> MHLMRACITFCIASTAVVAVNAALVAEDAPVLSKAFVDRVNRLNRGIWKAKYDGVMQNITLREAKRLNGVIKKNNNASILPKRRFTEEEARAPLPSSFDSAEAWPNCPTIPQIADQSACGSCWAVAAASAMSDRFCTMGGVQDVHISAGDLLACCSDCGDGCNGGDPDRAWAYFSSTGLVSDYCQPYPFPHCSHHSKSKNGYPPCSQFNFDTPKCNYTCDDPTIPVVNYRSWTSYALQGEDDYMRELFFRGPFEVAFDVYEDFIAYNSGVYHHVSGQYLGGHAVRLVGWGTSNGVPYWKIANSWNTEWGMDGYFLIRRGSSECGIEDGGSAGIPLAPNTA

The crystal structure of Trypanosoma brucei procathepsin B (TbCatB) in complex with its native propeptide represents the first novel bioinformation obtained by applying the SFX approach at a free-electron laser. This enzyme is of scientific and medical interest, since the knockout of its encoding gene has been shown to be lethal to the parasite that causes sleeping sickness in Africa, which turns TbCatB into an urgently required potential new drug target. TbCatB crystals grew spontaneously within living baculovirus-infected insect cells during protein overexpression to a size of 10–15 µm in the longest dimension.

By combining diffraction data from 80 Trypanosoma brucei procathepsin B crystals with an average volume of 9 µm3, a complete data set to 3.0 Å resolution has been assembled. Diffraction experiments were conducted on the P14 microfocus beamline at the PETRA III storage ring (DESY, Hamburg) with a 4 × 5 µm (FWHM) microfocus beam, a total photon flux of 1.2 × 1012 photons s−1 at the sample position and a photon energy of 10.00 keV. To collect a complete data set, we employed a data-collection strategy in which a region of interest of 600 × 600 µm was raster scanned with rotation exposures. After iterative merging and scaling, 109 661 reflection intensities in the resolution range from 88 to 3.0 Å were merged into a final data set consisting of 8881 merged reflection intensities with an overall completeness of 99.8%. This final set of reflection intensities included data from 426 diffraction patterns collected from 80 individual TbCatB crystals in 120 groups. During stepwise model building and refinement, 62 propeptide residues and five carbohydrate residues were manually placed in difference electron-density maps. No electron density is observed for nine flexible amino-acid side chains mainly located within a loop region spanning residues His195–Asn209 or for ten atoms of the carbohydrate structures. The superposition of the peptide backbone atoms of both structures revealed a high degree of consistency, resulting in an average r.m.s.d. value of 0.35 ± 0.19 Å, which is comparable to the overall coordinate error of 0.32 Å estimated based on maximum likelihood by REFMAC5.5. Main-chain deviations of more than 0.8 Å are limited to nine residues located at the N-terminus and C-­terminus, in flexible loop regions and at positions flanking the disordered part of the propeptide region that results from an increased flexibility of the residues after proteolytic cleavage between Ser78 and Ile79. Despite the overall similarity in atomic coordinates, systematic differences were observed in the relative heights of the electron-density peaks at the 12 Cys SG atoms involved in disulfide bridges.2-{[2-methoxy-4-(4-methylpiperazin-1-yl)phenyl]amino}-11-methyl-5-(2,2,2-trifluoroethyl)-5,11-dihydro-6H-pyrimido[4,5-b][1,4]benzodiazepin-6-one 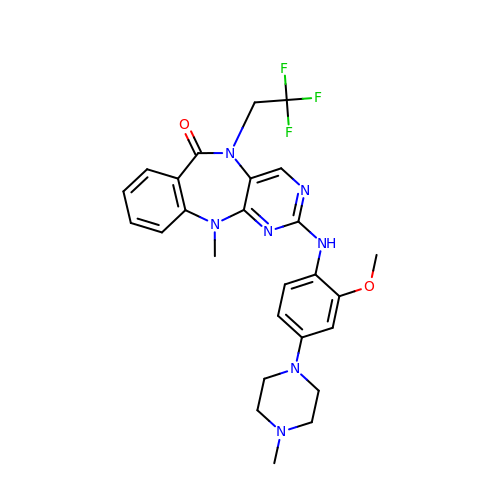| C26 H28 F3 N7 O2 | OQFCHSFVWSLDAO-UHFFFAOYSA-N> VEMVDNLRGKSGQGYYVEMTVGSPPQTLNILVDTGSSNFAVGAAPHPFLHRYYQRQLSSTYRDLRKGVYVPYTQGKWEGELGTDLVSIPHGPQVTVRANIAAITESDKFFIQGSNWEGILGLAYAEIARPDDSLEPFFDSLVKQTHVPNLFSLQLCGAGFPLQQSEVLASVGGSMIIGGIDHSLYTGSLWYTPIRREWYYEVIIVRVEINGQDLKMDCKEYNYDKSIVDSGTTNLRLPKKVFEAAVKSIKAASSTEKFPDGFWLGEQLVCWQAGTTPWNIFPVISLY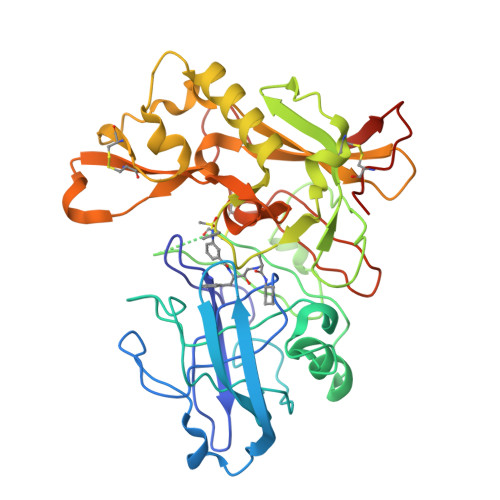LMGEVTQQSFRITILPQQYLRPVEDVATSQDDCYKFAISQSSTGTVMGAVIMEGFYVVFDRARKRIGFAVSACHVHDEFRTAAVEGPFVTLDMEDCGYNIPQTDE> MGSSHHHHHHSQDPMSLNLVSEQLLAANGLKHQDLFAILGQLAERRLDYGDLYFQSSYHESWVLEDRIIKDGSYNIDQGVGVRAISGEKTGFAYADQISLLALEQSAQAARTIVRDSGDGKVQTLGAVEHSPLYTSVDPLQSMSREEKLDILRRVDKVAREADKRVQEVTASLSGVYELILVAATDGTLAADVRPLVRLSVSVLVEEDGKRERGASGGGGRFGYEFFLADLDGEVRADAWAKEAVRMALVNLSAVAAPAGTMPVVLGAGWPGVLLHEAVGHGLEGDFNRRGTSVFSGQVGELVASELCTVVDDGTMVDRRGSVAIDDEGTPGQYNVLIENGILKGYMQDKLNARLMGMTPTGNGRRESYAHLPMPRMTNTYMLPGKSTPQEIIESVEYGIYAPNFGGGQVDITSDK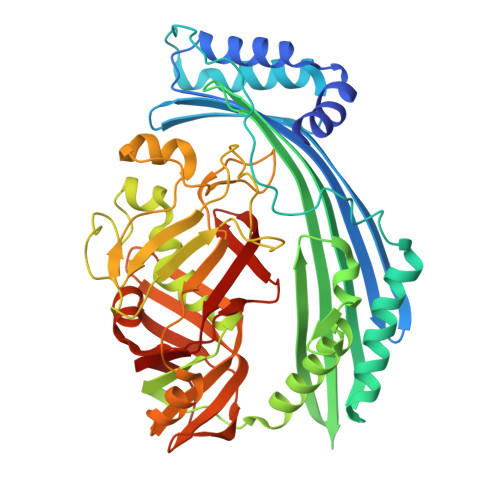FVFSTSEAYLIENGKVTKPVKGATLIGSGIETMQQISMVGNDLKLDNGVGVCGKEGQSLPVGVGQPTLKVDNLTVGGTA> MKTQVAIIGAGPSGLLLGQLLHKAGIDNVILERQTPDYVLGRIRAGVLEQGMVDLLREAGVDRRMARDGLVHEGVEIAFAGQRRRIDLKRLSGGKTVTVYGQTEVTRDLMEAREASGATTVYQAAEVRLHDLQGERPYVTFERDGERLRLDCDYIAGCDG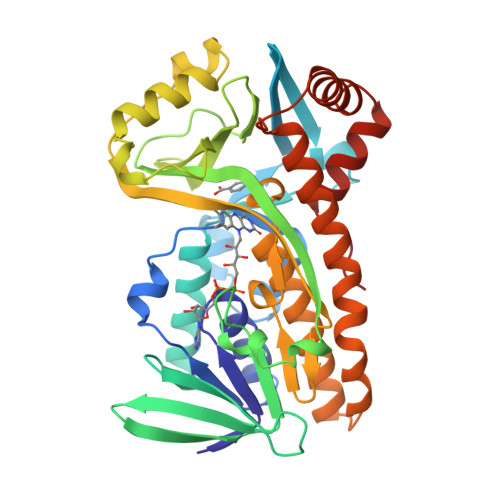FHGISSQSIPAERLKVFERVYPFGWLGLLADTPPVSHELIYANHPRGFALCSQRSATRSRYYVQVPLTEKVEDWSDERFWTELKARLPAEVAEKLVTGPSLEKSIAPLRSFVVEPMQHGRLFLAGDAAHIVPPTGAKGLNLAASDVSTLYRLLLKAYREGRGELLERYSAICLRRIWKAERFSWWMTSVLHRFPDTDAFSQRIQQTELEYYLGSEAGLATIAENYVGLPYEEIE> MGSHHHHHHMAAPRRTVVLAIDLQAGVTPGCFDEEGVLSRAAALVERARAGGVPVVWVHHDPVGVGTPEWELAAPLHRAEGEPLVRKNYRDSFADTTLRETLDELGATHLVITGAQSDFAVRTTMQRAAAEGYDVTLV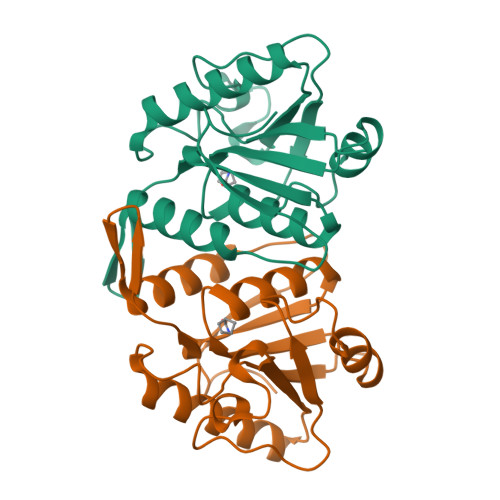SDAHTTVDTEWEGVRISGEQIVAHTNMYFSGLRYPGQEFVIATHDHVAL> SG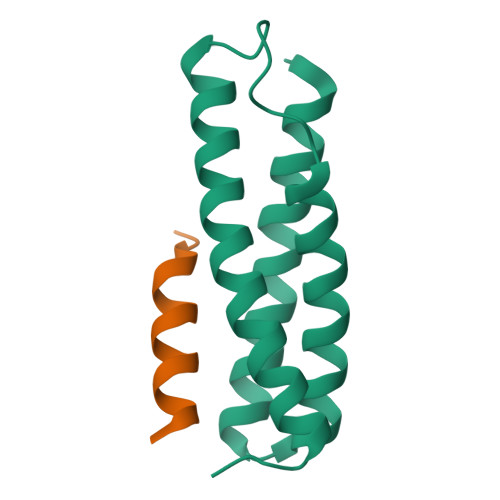EPAEIKIIREAYKKAFLFVNKGLNTDELGQKEEAKNYYKQGIGHLLRGISISSKESEHTGPGWESARQMQQKMKETLQNVRTRLEILEKGLAT;> STSASEDIDFDDLSRRFEELKKKTW To obtain sufficient iron, S. pneumoniae evolved two major highly conserved iron ABC transporters, which are termed Piu (for pneumococcal iron uptake) and Pia (for pneumococcal iron acquisition) systems, respectively. Pia system is responsible for the transport of hydroxamate siderophores such as ferrichrome and ferrioxamin B, whereas Piu system for the transport of heme from hemoglobin. The overall structure of PiaA is composed of an individual N-terminal and a C-terminal domain linked by an α-helix. The N- and C-terminal domains face each other to form a hydrophobic and plastic cleft.

The structures of Se-Met substituted apo-PiaA and ferrichrome-binding complex were subsequently solved at 2.7 Å and 2.1 Å, respectively, by molecular replacement. Each asymmetric unit of the apo-PiaA structure contains two molecules, which are quite similar to each other with an RMSD of 0.24 Å over 278 Cα atoms. Segments 1 (residues Asn84−Lys90) and 2 (residues Glu248−Glu252) at the entrance of this cleft are missing from the electron density map due to their high flexibility. Notably, Segments 1 and 2 are located at the N- and C-terminal domains, respectively, indicating the cooperativity between the two domains. Different from E. coli FhuD, the most N-terminus of apo-PiaA structure has an extended β-hairpin, which may function as a hinge to connect the N-terminal transmembrane α-helix that is inserted in the membrane of Gram-positive bacteria. Superposition of apo-PiaA and PiaA-B3P against the ferrichrome-complexed form gives an RMSD of 0.31 Å for 262 Cα atoms and 0.45 Å for 283 Cα atoms, respectively. Superposition of the complex against the apo-PiaA structure revealed that most residues in the binding cleft undergo subtle conformational changes, except for residues Asn83 and Tyr84 that locate at the invisible Segment 1 in the apo-form.

>MGHHHHHHMNSVKNEENTSKEHAPDKIVLDHAFGQTILDKKPERVATIAWGNHDVALALGIVPVGFSKANYGVSADKGVLPWTEEKIKELNGKANLFDDLDGLNFEAISNSKPDVILAGYSGITKEDYDTLSKIAPVAAYKSKPWQTLWRDMIKIDSKALGMEKEGDELIKNTEARISKELEKHPEIKGKIKGKKVLFTMINAADTSKFWIYTSKDPRANYLTDLGLVFPESLKEFESEDSFAKEISAEEANKINDADVIITYGDDKTLEALQKDPLLGKINAIKNGAVAVIPDNTPLAASCTPTPLSINYTIEEYLNLLGNACKNAK[2x]5-[5-(4-chloranyl-3-fluoranyl-phenyl)-4-methyl-pyrazol-1-yl]-2-phenylmethoxy-benzoic acid | C24 H18 Cl F N2 O3 | 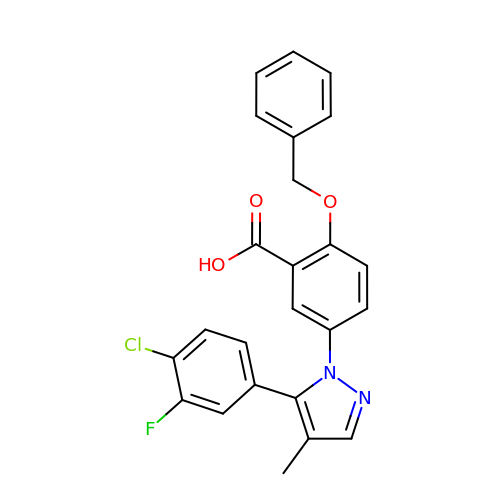NWWKXTLGLBRUHA-UHFFFAOYSA-N The nucleotide binding and leucine-rich repeat (NLR) class of intracellular immune receptors is an important component of innate immunity in plants and animals. The central domain, termed NB-ARC (nucleotide binding adaptor shared by APAF-1, plant R proteins, and CED-4) in plant NLRs, is a hallmark of this protein family and plays a key role as a molecular switch, mediating conformational changes required for activation. NB-ARC domains consist of a nucleotide binding domain (NB), a helical domain (HD1), and a winged helix domain (WHD). In these cases, one NLR acts as a pathogen sensor, requiring a second helper NLR to initiate immune signaling. Such is the case in the solanaceous NRC immune receptor network, which is composed of multiple sensor NLRs that require an array of downstream helper NLRs termed NRCs (NLRs required for cell death) to successfully initiate immune signaling.

To further define the interface between SS15 and NRC proteins, we attempted to crystallize SS15 in complex with the NB-ARC domain of several NRC proteins. We obtained crystals of SS15 in complex with the NB-ARC domain of SlNRC1, a tomato NRC that is inhibited by the nematode effector. Because purification and crystallization trials of SS15 in complex with NRC2NB-ARC and NRC3NB-ARC were unsuccessful, we moved forward with the SlNRC1NB-ARC-SS15 crystals. We propose that SS15 prevents conformational changes that are critical for NLR activation by binding and immobilizing the NB-HD1 hinge. By binding and immobilizing a critical hinge loop in the HD1 region of the NB-ARC, SS15 restricts movement of the NB domain relative to the HD1 and WHD domains, preventing immune receptor activation. Candidate residues (highlighted in red) were shortlisted on the basis of the interface identified in the co-crystal structure of SS15 and the SlNRC1 NB-ARC domain, as well as being conserved in SlNRC1, NRC2, and NRC3 but not NRC4 and AtZAR1. Combining information from the cocrystal structure and the alignments allowed us to select 13 candidate residues to test by mutagenesis in NRC2. We conclude that the E316 and D317 residues are critical for SS15-mediated inhibition of NRC2 and that mutating these residues to their equivalent amino acid in NRC4 allows Rx/CP-activated NRC2 to evade SS15 association and inhibition. Mutational studies of this interface allowed us to generate A amino acid variant of NRC2 (NRC2D317K) that evades SS15 inhibition without compromising receptor signaling capacity.

>GPPVVEEDDVVGFDDEAQTVIDRLLEGSGDLEVIPVVGMPGLGKTTLATKIFKHPKIEYEFFTRLWLYVSQSYKTRELYLNIISKFTGNTKHCRDMSEKDLALKVQEILEEGGKYLIVLDDVWSTDAWDRIKIAFPKNDKGNRVLLTTRDHRVARYCNRSPHDLKFLTDEESWILLEKRAFHKAKCLPELETNGKSIARKCKGLPLAIVVIAGALIGKSKTIKEWEQVDQSVGEHFINRDQPNSCDKLVRMSYDVLPYDWKACFLYFGTFPRGYLIPARKLIRLWIAEGFIQYRGDLSPECKAEEYLNELVNRNLVMVMQRTVDGQIKTCRVHDMLYEFCWQEATTE[2x];>[2x]GPSPKANAKLEKVPSGNAESTPVLTLQNRWAYSARDEKLAWDSAARDEKLELTEPAGLIVQFIGENSKHRSVRAKLPIPKGNSGIFYYEVTISGDGDAIYIGLATEQMPLRDTHVGYNEGTYGYGSSGKFWGHEVGGCSHWGNERPYIDGQPKFDRNNIIGCGVNLKTRQIIYTHNGRPLETTGLLVAESAAELYPCVSLFTSGNEIEANFGTKPFKFNIAEGI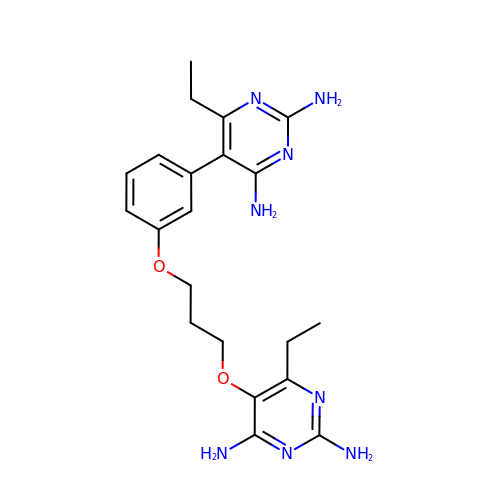5-(3-{3-[(2,4-diamino-6-ethylpyrimidin-5-yl)oxy]propoxy}phenyl)-6-ethylpyrimidine-2,4-diamine | C21 H28 N8 O2 | IMDBCJZTZFNOKU-UHFFFAOYSA-N> SHPAGIILTRDSYYTIPSM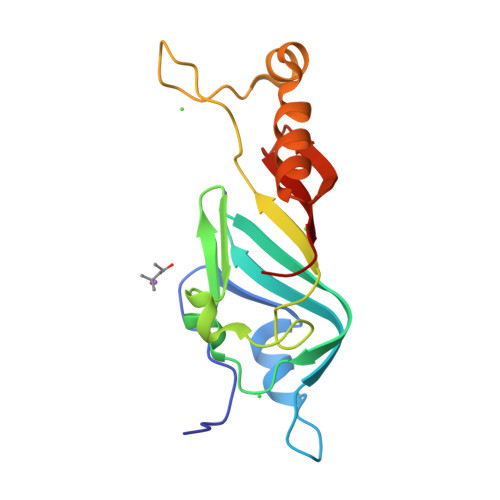EELARSVDENGECIVNGFTIGREGFGSIYFEGIVNLTNLDLDSIVHIRRKEVIVYVDDQNKPPLGEGLNRPAQVTLDEVWPIDKTSRCMITSPERLSEMNYKSKLENASRKQGAQFVDYRPESGSWVFKVNHF Malonyl-CoA reductase (MCR) is a NADPH-dependent bi-functional enzyme that performs alcohol dehydrogenase and aldehyde dehydrogenase (CoA-acylating) activities in the N- and C-terminal fragments, respectively. It catalyzes the two-step reduction of malonyl-CoA to 3-hydroxypropionate (3-HP), a key reaction in the autotrophic CO2 fixation cycles of Chloroflexaceae green non-sulfur bacteria and the archaea Crenarchaeota. In contrast, green non-sulfur bacteria, including members of the genera Chloroflexus and Roseiflexus, employ a single bi-functional MCR to catalyze both reduction reactions of malonyl-CoA. Full-length RfxMCR was a homodimer of two cross-interlocked subunits, each containing four tandemly arranged short-chain dehydrogenase/reductase (SDR) domains.

The crystal structure of RfxMCR-N in complex with NADP+–MSA was determined by the molecular replacement method and reﬁned to an Rwork of 19.62% and an Rfree of 20.81% at 2.0 Å resolution. Although the P6522 crystal contained only a monomer RfxMCR-N in one asymmetric unit, it was packed into a homodimer in the crystal. Although SDR1 (Met1–Pro292) and SDR2 (Thr293–Gly572) in RfxMCR-N had identical architectures, only SDR1, which contained the conserved Tyr-X-X-X-Lys motif, was resolved with NADP+ bound. Surprisingly, we observed an extra electron density that precisely matched the reduction intermediate MSA near the nicotinamide ring of NADP+. The carboxyl groups of MSA were immobilized by hydrogen bonding interactions with Tyr172 (2.6 Å), Arg175 (2.7 Å), and Tyr178 (2.9 Å), whereas the aldehyde group was hydrogen bonded with the hydroxyl group of Thr165 (2.9 Å). The nicotinamide ring was stabilized by a hydrogen bond with Ser213 (3.2 Å), and the ribose oxygen formed a hydrogen bond with the amino nitrogen of Lys182 (2.7 Å). Specifically, the side chains of Arg41 and Asp70 in SDR1 were flipped by ~7.2 Å and 9.3 Å, respectively, to stabilize the NADP+ adenine ring. Especially, the α10 helix (Ser213–Gly228) was rotated by ~20° toward the substrate-binding pocket to cover MSA and the NADP+ nicotinamide ring. This resulted in the closure of the MSA-binding site and shrinking of the substrate-binding pocket. In the structure of NADP+–MSA-bound RfxMCR-N, Thr165 stabilized the reaction intermediate MSA by forming hydrogen bonds with the C3 carbonyl oxygen, which facilitates nucleophilic attack by the NADPH hydride on the C3 atom of MSA.

> MMSTVRRLEGKVALITGGAGNIGEVITRRFLAEGATVVITGRNAEKLAVYRRRLIDEERVAPERVVALRMDGSDIAQVRAGVAQIVHGGTDVPIPLHRIDILVNNAGSAGPRRRLVDIPLEPSEVQPPDSETLAQAVGNLVGITWNLTRAAAPHMPSGSSVINISTIFSRTDYYGRIAYVAPKAALNALSDGLARELGVRGIRVNTIYPGPIESERIYTMFQAMDALKGQPEGDTASGFLRMMRLSRIDQNGEVVKRFPSPVDVANTAVFLASDESAAFTGHAFEVTHGMEVPTESRTTFVSRPGLRSVDATGKVILICAGDQVDDAVALADTLRSCRATVVIGFRDPRALEKASVLLREPRHALAADMYGRPTMTAEARLVRLDPLDPRAAAQTLEQIHAELGAIHHAVVLPGQSRHAPSASLIEVDDQVVERFLHQELVGTIALARELARFWEEYPSGSSMHRVLFVSNPDDQQGNQYSHILRAAVEQLVRVWRHESEYDSVNPAHQQEGQSSAAVWANQLIRYVNNEMANLDFTCAWVAKLLGSDRRIAEINLYLPEEIVGTIGVHNPGFHHHHHH>SNAMALKYPSGKEYRGNKPNAARRPAADYANRGMTLEDDLNATNEYYRERGIAVIHKKPTPVQIVRVDYPKRSAAVITEAYFRQASTTDYNGVYRGKYIDFEAKETKNKTAFPLKNFHAHQIRHMEQVVAHGGICFAILRFSLLNETYLLDASHLIAWWNK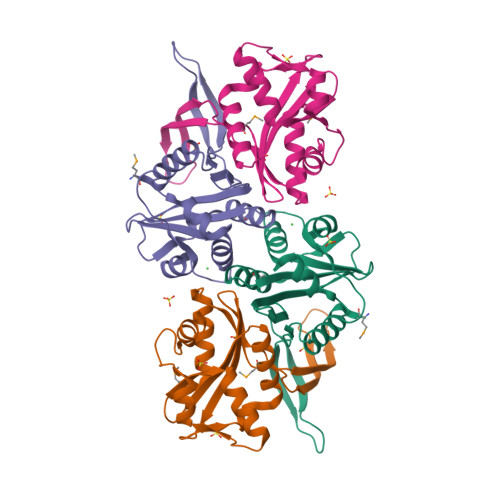QEAGGRKSIPKQEIERHGHSIPLGYQPRLDYISVVDNVYFTR[4x]>[5x]MAHHHHHHMKLVKTPLKDCYIIEPTVFEDERGYFYEKYNEKKFEELTGLNGHFVQDNISKSSYGVLRGLHLQKGKHAQAKLVSCLEGRV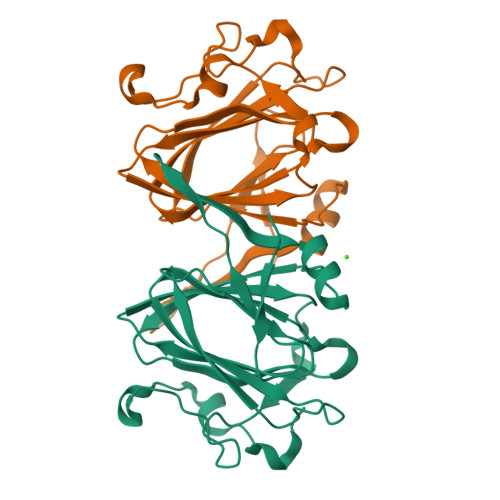WDVAVDLRENSETFGKCYGMELSAENKLQFYVPRGFAHGFVVLSETAVFSYKCDNFYNKESEGSVKFNDSDLSIDWKIPEADMILSEKDQNAPAFKDKNY>KMAFTLADRVTEEMLADKAALVVEVVEENYHDAPIVGIAVVNEHGRFFLRPETALADPQFVAWLGDETKKKSMFDSKRAAVALKWKGIELCGVSFDLLLAAYLLDPAQGVDDVAAAAKMKQYEAVRPDEAVYGKGAKRAVPDEPVLAEHLVRKAAAIWELERPFLDELRRNEQDRLLVELEQPLSSILAEMEFAGVKVDTKRLEQMGKELAEQLGTVEQRIYELAGQEFNINSPKQLGVILFEKLQLPVLKKTKTGYSTSADVLEKLAPYHEIVENILHYRQLGKLQSTYIEGLLKVVRPATKKVHTIFNQALTQTGRLSSTEPNLQNIPIRLEEGRKIRQAFVPSESDWLIFAADYSQIELRVLAHIAEDDNLMEAFRRDLDIHTKTAMDIFQVSEDEVTPNMRRQAKAVNYGIVYGISDYGLAQNLNISRKEAAEFIERYFESFPGVKRYMENIVQEAKQKGYVTTLLHRRRYLPDITSRNFNVRSFAERMAMNTPIQGSAADIIKKAMIDLNARLKEERLQAHLLLQVHDELILEAPKEEMERLCRLVPEVMEQAVTLRVPLKVDYHYGSTWYDAK[2x]

Polymerases generate nascent strands of genetic material by stepwise phosphoryl transfer of nucleotides to primer termini, yielding O3′→P5′ phosphodiester linkages. We reported that 3′-NH2 primer extension can be catalyzed by a modified DNA polymerase, yielding N3′→P5′ phosphoramidate DNA (NP-DNA). The large fragment of DNA polymerase I (BF), cloned from the thermophilic soil bacterium Geobacillus stearothermophilus (Bst), acquires nontrivial levels of N3′→P5′ polymerase activity via two surprisingly minor substitutions: (A) a single active site mutation (F710Y) and (B) substitution of its divalent Mg2+ cofactors with Ca2+ (1). To add evidence that a single divalent metal ion cofactor catalyzes unnatural NP synthesis in BF, a polymerase A family member, we carried out a single nucleotide primer extension reaction in intact crystals.

We crystallized active substrate-bound BF polymerase F710Y/D598A with a 3′-amino terminal DNA primer and DNA template in the presence of Ca2+ and 2′-deoxyguanosine 5′-triphosphate (dGTP). Reactions were then initiated in the intact crystals by pH-shift from an acidic mother liquor (pH < 6) to a basic soaking liquor at pH 8.8, and reacting crystals were quenched at various times by flash freezing. By scaling reflections from 19 total crystals (resolution 2.0 – 2.7 Å) across the time course (0 – 24 h), we could estimate voxel-wise first-order rate constants for changes in real-space electron density across the asymmetric unit and particularly at the reaction center. By following the reaction at subsequent times, we observed monotonic accumulation of nascent NP bond density between the primer terminal 3′-amino group and the substrate α-phosphate with concomitant loss of electron density between the α- and β-phosphates with similar first-order rate constants. Conformational changes in both the upstream and downstream nucleotides flanking the nascent bond are linearly correlated with covalent bonding. Unlike for native phosphodiester catalysis, only a single metal ion cofactor is detectable by crystallography during NP catalysis. The lack of electron density for an A-site metal ion in the ground state and at later time points is also consistent with the expectation of a neutral nucleophile in the NP reaction and the generally weak affinity of aliphatic amines for Ca2+.Herein we present the development of a PluriZyme, TR2E2, with efficient native transaminase (k cat: 69.49±1.77 min−1) and artificial esterase (k cat: 3908–0.41 min−1) activities integrated into a single scaffold, and evaluate its utility in a cascade reaction. The reaction proceeds through the conversion of the β‐keto ester into the β‐keto acid at the hydrolytic site and subsequently into the β‐amino acid (e.e. >99 %) at the transaminase site. In addition, we report the crystal structures of the TR2 enzyme and the newly designed TR2E2 PluriZyme. It presents the typical type I fold of class III ω‐TA observed in known structures present in the PDB database, and it contains the characteristic pyridoxal‐5′‐phosphate (PLP)‐binding domain composed of β‐sheets and the catalytic base Lys289.

Diffracting crystals were obtained for TR2E2 as well. Datasets for each crystal were collected and refined to a resolution of 3.3 Å. Only purified TR2E2, which retained approximately 80 % of the original transaminase activity (k cat: 69.48±1.77 min−1), was capable of hydrolyzing pNPA, pNPP, and pNPB, with the latter being the preferred substrate (k cat: 0.41±0.05 min−1). This variant contains two mutations, A172S and Q173H. The artificial esterase catalytic triad was observed in the TR2E2 crystal structures and is composed of Ser172 and His173 of chain A (magenta) and Glu317 of chain B (green); similar to the transaminase's active site, the esterase site is composed of a functional protein dimer. The RMSD between TR2 and TR2E2 was calculated to be 0.71 Å between 299 of 389 C_α atoms of the aligned residues, indicating that no large conformational change occurs due to mutations, as also confirmed by the transaminase activity assay. Notably, the distance between both active sites is ≈20 Å, with the esterase site being more solvent‐exposed and located at the beginning of the tunnel and the transaminase site being more buried in the protein structure. Structural analysis revealed a 20 Å distance between both active sites, with the esterase site being solvent‐exposed and the transaminase site buried in the protein structure, thus ensuring that the transfer of the reaction intermediate within the protein structure is theoretically possible. When the residues Ser172 and His173 were replaced with Ala, the activity was completely abolished. Thus, the insertion of the hydrolytic site helped stabilize this region by adding two internal hydrogen bonds, improving the thermostability of the enzyme. The finding that both TR2 and TR2E2 retained high activity at 50–65 °C was consistent with their denaturation temperatures (56.23±0.09 °C and 61.85±0.11 °C, respectively), as revealed by circular dichroism spectroscopy.

>MSQSQRSTADWQRLDAAHHLHPFTDYGELNTKGSRIITRAEGCYLWDSDGNQILDGMAGLWCVNIGYGRKELAEVAYRQMQELPYYNNFFQCSHPPAIELSRLLSEVTPKHMNHVFFTGSGSDSNDTILRMVRYYWKLLGKPYKKVVISRENAYHGSTVAGASLSGMKAMHSHGDLPIPGIEHIEQPYHFGRAPDMDPAEFGRQAAQALERKIDEIGECNVAAFIAEPIQGAGGVIIPPDSYWPEIKRICAERDILLIVDEVITGFGRLGTWFGSQYYDLQPDLMPIAKGLSSGYMPIGGVMVSDRVAKVVIEEGGEFFHGYTYSGHPVAAAVAAENIRIMRDEGIIERAGAEIAPYLQARWRELGEHPLVGEARGVGMVAALELVKSKQPLERFEEPGKVGSLCRDLSVKNGLVMRAVGGTMIISPPLVLSREQVDELIDKARRTLDETHKAIGGALEHHHHHH[4x]> GSPEAE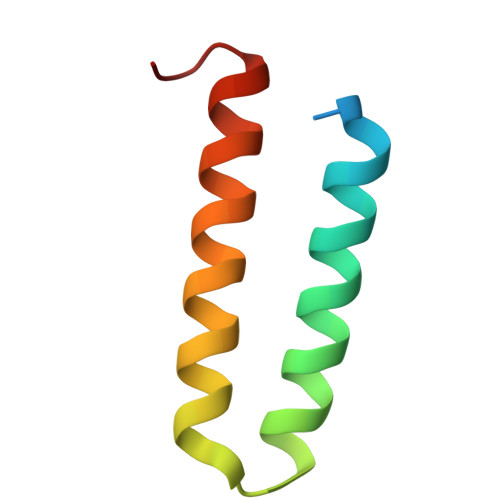EPIEEELLLQQIDNIKAYIFDAKQCGRLDEVEVLTENLRELKHTLAKQKGGTD>[2x]MAFKLPNLPYAYDALEPYIDQRTMEFHHDKHHNTYVTKLNATVEGTELEHQSLADMIANLDKVPEAM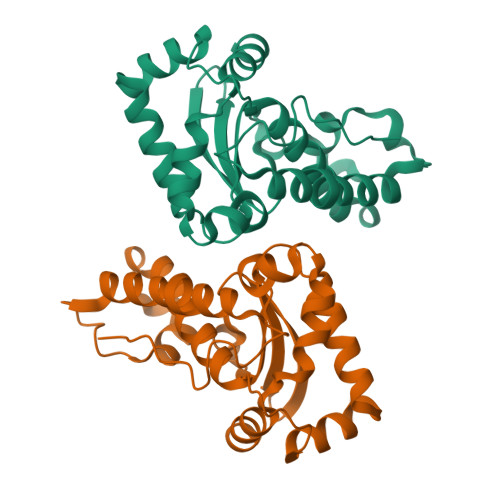RMSVRNNGGGHFNHSLFWEILSPNSEEKGGVIDDIKAQWGTLDEFKNEFANKATTLFGSGWTWLVVNDGKLEIVTTPNQDNPLTEGKTPILLFDVWEHAYYLKYQNKRPDYMTAFWNIVNWKKVDELYQAAK>MSCGDAKLNHPAPDFNETALMPNGTFKKVALTSYKGKWLVLFFYPMDFTFVCPTEICQFSDRVKEFSDIGCEVLACSMDSEYSHLAWTSIERKRGGLGQMNIPILADKTKCIMKSYGVLKEEDGVAYRGLFIIDPKQNLRQITVNDLPVGRDVDEALR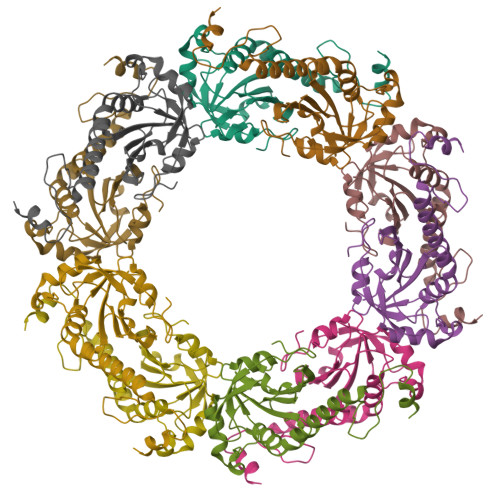LVKAFQFVEKHGEVCPANWKPGDKTMKPDPEKSKEYFGA[10x]Nonribosomal peptides (NRPs) represent a valuable source of clinical therapeutics. These natural products are biosynthesized by multifunctional enzymatic assembly lines, called nonribosomal peptide synthetases (NRPSs), that use dedicated modules to incorporate each building block selectively and sequentially into the peptide scaffold. NRPS modules typically possess three core domains, which perform substrate selection and activation (adenylation or A domains), shuttling of activated substrates (thiolation or T domains, also called peptide carrier proteins, PCP or CP domains) and peptide bond formation (condensation or C domains), respectively. The enzymatic assembly line that produces the microbial lipopeptide antibiotic surfactin, surfactin synthetase, consists of the following three proteins: trimodular SrfA-A, trimodular SrfA-B and monomodular SrfA-C. The modules are composed of several functional domains, including C, A and T domains. In the current study, we re-engineered the donor substrate specificity of the SrfA-C C domain (green) to enable direct acylation of the acceptor Leu (residue 7, yellow highlight) with a fatty acid rather than an amino acid.

We also undertook crystallization of the C domain covalently fused to the upstream donor complex, the 10-undecynoyl-NH-ppant-T domain, but crystals of the didomain did not grow. However, we also solved the high-resolution structures of wild-type SrfA-C, and comparison with SrfA-CFA structures provides insight into the origins of the specificity shift. Although the terminal C domain in surfactin synthetase is known to tolerate some changes in its native peptide substrate, we sought to expand its substrate scope to nonpeptidyl acyl donors. To first test whether SrfA-C has any latent activity with inherently less reactive fatty acids, we examined its ability to process 10-undecynoic acid, which contains a terminal alkyne for bioorthogonal labeling. Although activity was detected, the fatty acid was processed >15 times more slowly than O-propargyl-Tyr. The lipid substrate of RzmA-Cs sits deep within a pocket in the N-terminal lobe of the C domain, and comparison of the structures suggested that expansion of the SrfA-C substrate pocket between the core β-sheet in the N-terminal lobe and the fourth α-helix, close to the active site, might improve 10-undecynoic acid recognition. We therefore prepared a large combinatorial library in which hydrophobic (Ile39, Met41, Trp143, Tyr145, Phe155 and Val159) and negatively charged (Glu37) residues lining this site were simultaneously randomized using degenerate codons that code for small and hydrophobic amino acids. Structure-based considerations would certainly have included mutation of Glu37 to a smaller residue, as the side chain of Glu37 blocks the fatty acid pocket in all crystal structures.

> MHHHHHHHHPDLGTGSENLYFQGAMADQVQDMYYLSPMQEGMLFHAILNPGQSFYLEQITMKVKGSLNIKCLEESMNVIMDRYDVFRTVFIHEKVKRPVQVVLKKRQFQIEEIDLTHLTGSEQTAKINEYKEQDKIRGFDLTRDIPMRAAIFKKAEESFEWVWSYHHIILDGWCFGIVVQDLFKVYNALREQKPYSLPPVKPYKDYIKWLEKQDKQASLRYWREYLEDFEGQTTFAEQRKKQKDGYEPKELLFSLPEAETKAFTELAKSQHTTLSTALQAVWSVLISRYQQSGDLAFGTVVSGRPAEIKGVEHMVGLFINVVPRRVKLSEGITFNDLLKQLQEQSLQSEPHQYVPLYDIQSQADQPKLIDHIIVFENYPLQDAKNEESSENGFDMVDVHVFEKSNYDLNLMASPGDEMLIKLAYNENVFDEAFILRLKSQLLTAIQQLIQNPDQPVSTINI Nonribosomal peptide synthetases (NRPSs) produce small peptides as secondary metabolites in fungi and bacteria. Tomaymycin is synthesized in Streptomyces and Micrococci by an NRPS consisting of the initiation module TomA and the elongation/termination module TomB. TomB contains a C domain (BC; TomB91–533), an A domain (BA; TomB534–1055), which functions to load the ppant arm of its PCP domain (BPCP; TomB1056–1141) with 4-ethylidene proline, and a reductase domain (BR; TomB1142–1535). The C domain binds two substrate-loaded PCPppant domains—termed the donor and acceptor PCPs—and transfers the growing peptide chain from the donor PCP of the upstream module onto the aminoacyl subunit carried by the acceptor PCP of the same module.

The crystallization construct comprised residues 1 to 533; however, the first 79 residues did not yield resolvable electron density, resulting in crystal structures of only the BC domain (91 to 533) and the preceding 11 amino acids. (A) Crystallographic structure of BN-BC at 1.7-Å resolution (N-form). As other canonical C domains, TomB80–533 consists of N-terminal and C-terminal lobes, which adopt a chloramphenicol acetyltransferase fold and are arranged in a V shape. The N- and the C-lobes are shown in light and dark green, respectively. Two crossover elements extend from the C-terminal to the N-terminal lobe: the “floor” loop between β8 and β9 and the “latch” loop between β10 and β11. The two cross-over elements—the floor loop and latch loop—are shown in red and beige, respectively. Also highlighted in red is the junction between the N- and C-lobes. The catalytic tunnel is at the interface between the two lobes and includes the conserved motif 222HHXXXD227, where H223 is fundamental for catalysis. In both crystal forms, the catalytic tunnel of BC is wide enough to accommodate the ppant arm and their substrates at both the donor and acceptor sites. The tunnel is ~38 Å long with a minimum width of ~1.4 Å at the bottleneck, as measured by CAVER 3.0 (29).

> GPMLMNSPLRTTVLDLARTTLGSADLTAHEPLADRCEHPALLDDLATTLTAVFAVEITGADLAAGATVADVAARMDDRRDAPRIPELRAGLAPRDGRAVEASFGQSGIWLIDQYLPNPAAYNGPFFVRLPFSADPDRLHAAVRGVLRRQEVLRTTYALSDGTLRQNVSRDDDAVVFEVARYGDDKELDALVHRVANLRLDLARGPVIAVTCALGPANRSAVICNIHHIASDAASAGVFLRELLDAYDRLGRGLPVEADPLRPTYGDFSQWYRELMNPEALTRSLDHFAARLAGELPVLDLPTDRPRPPVKQHRGGTLPLHLPAAAADDFEALARTEGVTLFMALVAAYAVFLSRHTGQRRVLIGSPVSLRDDPATHELIGYFVNLVVLQQEIDDRMTVRDVLRRAREEVSEALRHKWAPFDKVVERLQPPRSSGYTPLVQTMLVLTQGDAGRISHDDTELRIERGAAHGAKYDLSLVFERDSEGLHGLIEYDADLFDEPTVRAMGDRLRHLMEQFARRPDAPLHELEALGAQERRSV4-methoxy-~{N}-oxidanyl-3-(2-phenylethanoylamino)benzamide 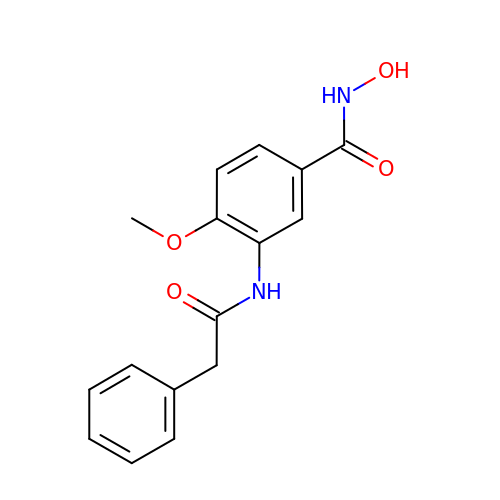| C16 H16 N2 O4 | DFZIVCDTMKHRDI-UHFFFAOYSA-N>GPGYQDPLTINADLQRVAEESLNAAVKRVGGVWGSAAVLEIGTGRLLALAPGGTRSVSAIYEPGSVGKLVTLAAAIDQKKVTPTSTFTVSSTRDMPNGERISDDSPHETQDMTVAGIIAHSYNTGTVQIGDTVSDSVRYEYMQKFGWGAKTGITLPSEESGILRPHTEWGDRDHYTTMFGQGVAVTTIQLAQMVAVFGQKGVLIPPRIIDGYDDENGVYTPTVMGESRQVVSEDTAQTVLNIMQGATQPGGTAEGIGAVKGYNVAAKTGTAENVGSSGSLTDTAATFTALIPAENPKIAVAVVIYKENGTVYGSTASAPVFVDIAQFAMREMKIPPSTVPLYKYPW[2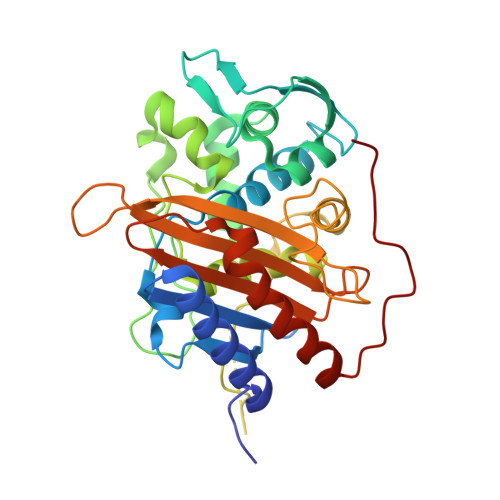x]> SANEDMPVERILEAELAVEPKTETYVEANMGLNPSSPNDPVTNICQAADKQLFTLVEWAKRIPHFSELPLDDQVILLRAGWNELLIASFSHRSIAVKDGILLATGLHVHRNSAHSAGVGAIFDRVLTELVSKMRDMQMDKTELGCLRAIVLFNPDSKGLSNPAEVEALREKVYASLEAYCKHKYPEQPGRFAK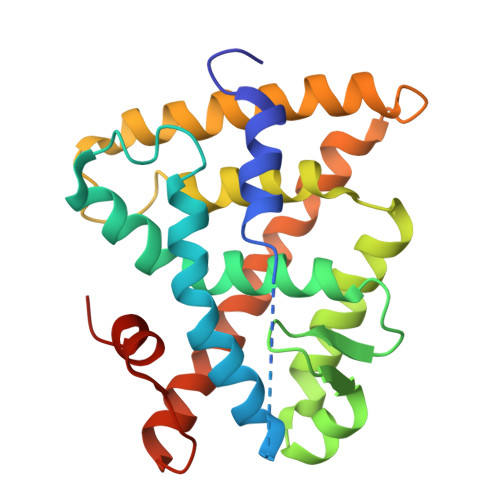LLLRLPALRSIGLKCLEHLFFFKLIGDTPIDTFLMEMLEAPHQMT> TEFLKPRLVDIEQVSSTHAKVTLEPLERGFGHTLGNALRRILLSSMPGCAVTEVEIDGVLHEYSTKEGVQEDILEILLNLKGLAVRVQGKDEVILTLNKSGIGPVTAADITHDGDVEIVKPQHVICHLTDENASISMRIKVQRGRGYVPASTRIHSEEDERPIGRLLVDACYSPVERIAYNVEAARVEQRTDLDKLVIEMETNGTIDPEEAIRRAATILAEQLEAFVDLRDVRQPEVKEEKPEFDPILLRPVDDLELTVRSANCLKAEAIHYIGDLVQRTEVELLKTPNLGKKSLTEIKDVLASRGLSLGMRLENW;> TEFLKPRLVDIEQVSSTHAKVTLEPLERGFGHTLGNALRRILLSSMPGCAVTEVEIDGVLHEYSTKEGVQEDILEILLNLKGLAVRVQGKDEVILTLNKSGIGPVTAADITHDGDVEIVKPQHVICHLTDENASISMRIKVQRGRGYVPASTRIHSEEDERPIGRLLVDACYSPVERIAYNVEAARVEQRTDLDKLVIEMETNGTIDPEEAIRRAATILAEQLEAFVDLRDVRQPEVKEEKPEFDPILLLPVDDLELTVRSANCLKAEAIHYIGDLVQRTEVELLKTPNLGKKSLTEIKDVLASRGLSLG;> VYSYTEKKRIRKDFGKRPQVLDVPYLLSIQLDSFQKFIEQDPEGQYGLEAAFRSVFPIQSYSGNSELQYVSYRLGEPVFDVQECQIRGVTYSAPLRVKLRLVIYEREAPEGTVKDIKEQEVYMGEIPLMTDNGTFVINGTERVIVSQLHRSPGVFFDSDKGKTHSSGKVLYNARIIPYRGSWLDFEFDPKDNLFVRIDRRRKLPATIILRALNYTTEQILDLFFEKVIFEIRDNKLQMELVPERLRGETASFDIEANGKVYVEKGRRITARHIRQLEKDDVKLIEVPVEYIAGKVVAKDYIDESTGELICAANMELSLDLLAKLSQSGHKRIETLFTNDLDHGPYISETLRVDPTNDRLSALVEIYRMMRPGEPPTREAAESLFENLFFSEDRYDLSAVGRMKFNRSLLREEIEGSGILSKDDIIDVMKKLIDIRNGKGEVDDIDHLGNRRIRSVGEMAENQFRVGLVRVERAVKERLSLGDLDTLMPQDMINAKPISAAVKEFFGSSQLSQFMDQNNPLSEITHKRRISALGPGGLTRERAGFEVRDVHPTHYGRVCPIETPEGPNIGLINSLSVYAQTNEYGFLETPYRKVTDGVVTDEIHYLSAIEEGNYVIAQANSNLDEEGHFVEDLVTCRSKGESSLFSRDQVDYMDVSTQQVVSVGASLIPFLEHDDANRALMGANMQRQAVPTLRADKPLVGTGMERAVAVDSGVTAVAKRGGVVQYVDASRIVIKVNEDEMYPGEAGIDIYNLTKYTRSNQNTCINQMPCVSLGEPVERGDVLADGPSTDLGELALGQNMRVAFMPWNGYNFEDSILVSERVVQEDRFTTIHIQELACVSRDTKLGPEEITADIPNVGEAALSKLDESGIVYIGAEVTGGDILVGKVTPKGETQLTPEEKLLRAIFGEKASDVKDSSLRVPNGVSGTVIDVQVFTRDGVEKDKRALEIEEMQLKQAKKDLSEELQILEAGLFSRIRAVLVAGGVEAEKLDKLPRDRWLELGLTDEEKQNQLEQLAEQYDELKHEFEKKLEAKRRKITQGDDLAPGVLKIVKVYLAVKRRIQPGDKMAGRHGNKGVISKINPIEDMPYDENGTPVDIVLNPLGVPSRMNIGQILETHLGMAAKGIGDKINAMLKQQQEVAKLREFIQRAYDLGADVRQKVDLSTFSDEEVMRLAENLRKGMPIATPVFDGAKEAEIKELLKLGDLPTSGQIRLYDGRTGEQFERPVTVGYMYMLKLNHLVDDKMHARSTGSYSLVTQQPLGGKAQFGGQRFGEMEVWALEAYGAAYTLQEMLTVKSDDVNGRTKMYKNIVDGNHQMEPGMPESFNVLLKEIRSLGINIELEDE;> EEFDAIKIALASPDMIRSWSFGEVKKPETINYRTFKPERDGLFCARIFGPVKDYECLCGKYKRLKHRGVICEKCGVEVTQTKVRRERMGHIELASPTAHIWFLKSLPSRIGLLLDMPLRDIERVLYFESYVVIEGGMTNLERQQILTEEQYLDALEEFGDEFDAKMGAEAIQALLKSMDLEQECEQLREELNETNSETKRKKLTKRIKLLEAFVQSGNKPEWMILTVLPVLPPDLRPLVPLDGGRFATSDLNDLYRRVINRNNRLKRLLDLAAPDIIVRNEKRMLQEAVDALLDNGRRGRAITGSNKRPLKSLADMIKGKQGRFRQNLLGKRVDYSGRSVITVGPYLRLHQCGLPKKMALELFKPFIYGKLELRGLATTIKAAKKMVEREEAVVWDILDEVIREHPVLLNRAPTLHRLGIQAFEPVLIEGKAIQLHPLVCAAYNADFDGDQMAVHVPLTLEAQLEARALMMSTNNILSPANGEPIIVPSQDVVLGLYYMTRDCVNAKGMVLTGPAERLYRSGLASLHARVKVRITEYEKDANGELVAKTSLKDTTVGRAILWMIVPKGLPYSIVNQALGKKAISKMLNTCYRILGLKPTVIFADQIMYTGFAYAARSGASVGIDDMVIPEKKHEIISEAEAEVAEIQEQFQSGLVTAGERYNKVIDIWAAANDRVSKAMMDNLQTETVINRDGQEEKQVSFNSIYMMADSGARGSAAQIRQLAGMRGLMAKPDGSIIETPITANFREGLNVLQYFISTHGARKGLADTALKTANSGYLTRRLVDVAQDLVVTEDDCGTHEGIMMTPVIEGGDVKEPLRDRVLGRVTAEDVLKPGTADILVPRNTLLHEQWCDLLEENSVDAVKVRSVVSCDTDFGVCAHCYGRDLARGHIINKGEAIGVIAAQSIGEPGTQLTMRTFHIGGAASRAAAESSIQVKNKGSIKLSNVKSVVNSSGKLVITSRNTELKLIDEFGRTKESYKVPYGAVLAKGDGEQVAGGETVANWDPHTMPVITEVSGFVRFTDMIDGQTITRQTDELTGLSSLVVLDSAERTAGGKDLRPALKIVDAQGNDVLIPGTDMPAQYFLPGKAIVQLEDGVQISSGDTLARIPQESGGTKDITGGLPRVADLFEARRPKEPAILAEISGIVSFGKETKGKRRLVITPVDGSDPYEEM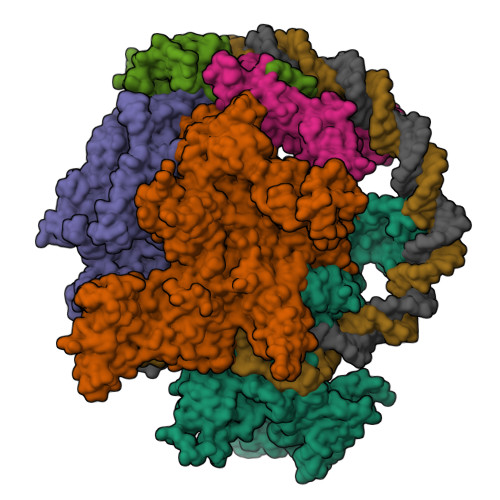IPKWRQLNVFEGERVERGDVISDGPEAPHDILRLRGVHAVTRYIVNEVQDVYRLQGVKINDKHIEVIVRQMLRKATIVNAGSSDFLEGEQVEYSRVKIANRELEANGKVGATYSRDLLGITKASLATESFISAASFQETTRVLTEAAVAGKRDELRGLKENVIVGRLIPAGTGYAYHQDRMRRRAAG;> ARVTVQDAVEKIGNRFDLVLVAARRARQMQVGGKDPLVPEENDKTTVIALREIEEGLINNQILDVRERQEQQEQEAAELQAVTAIAEGRR;> QLKLLVTRGKEQGYLTYAEVNDHLPEDIVDSDQIEDIIQMINDMGIQVMEEAPDADDLMLAENTADEDAAEAAAQVLSSVESEIGRTTDPVRMYMREMGTVELLTREGEIDIAKRIEDGINQVQCSVAEYPEAITYLLEQYDRVEAEEARLSDLITGFVDPNAENSIDPELAREKFAELRAQYVVTRDTIKAKGRSHATAQEEILKLSEVFKQFRLVPKQFDYLVNSMRVMMDRVRTQERLIMKLCVEQCKMPKKNFITLFTGNETSDTWFNAAIAMNKPWSEKLHDVSEEVHRALQKLQQIEEETGLTIEQVKDINRRMSIGEAKARRAKKEMVEANLRLVISIAKKYTNRGLQFLDLIQEGNIGLMKAVDKFEYRRGYKFSTYATWWIRQAITRSIADQARTIRIPVHMIETINKLNRISRQMLQEMGREPTPEELAERMLMPEDKIRKVLKISMETPIGDDEDSHLGIDFIEDTTSATTESLRAATHDVLAGLTAREAKVLRMRFGIDMNTDYTLEEVGKQFDVTRERIRQIEAKALRKLRHPSRSEVLRSFLDD> ELTPDQQTLLHFIMDSYNKQRMPQEITNKILKEEFSAEENFEILTEMATNHVQVLVEFTKKLPGFQTLDHEDQIALLKGSAVEA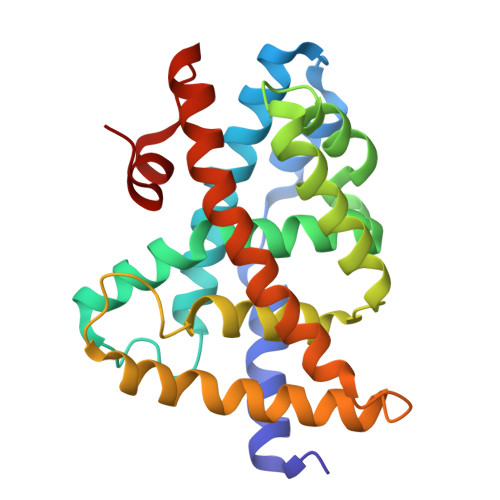MFLRSAEIFNKKLPSGHSDLLEERIRNSGISDEYITPMFSFYKSIGELKMTQEEYALLTAIVILSPDRQYIKDREAVEKLQEPLLDVLQKLCKIHQPENPQHFAELLGRLTELRTFNHHHAEMLMSWRVNDHKFTPLLEEIWDVQ>[2x]G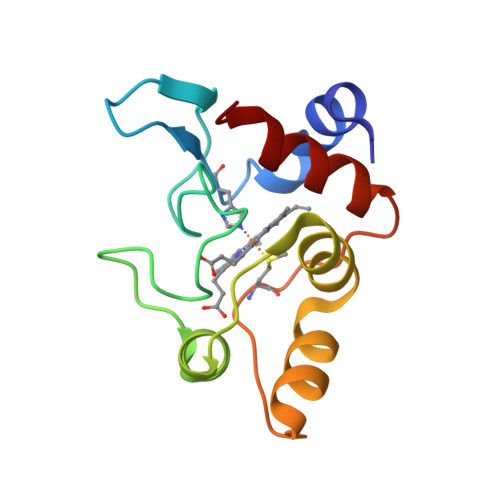DAAKGEKEFNKCKTCHSIIAPDGTEIVKGAKTGPNLYGVVGRTAGTYPEFKYKDSIVALGASGFAWTEEDIATYVKDPGAFLKEKLDDKKAKTEMAFKLAKGGEDVAAYLASVVK> GPLGSMEQTEVLKPRTLADLIRILHQLFAGDEVNVEEVQAIMEAYESDPTEWAMYAKFDQYRYTRNLVDQGNGKFNLMILCWGEGHGSSIHDHTNSHCFLKMLQGNLKETLFAWPDKKSNEMVKKSERVLRENQCAYINDSIGLHRV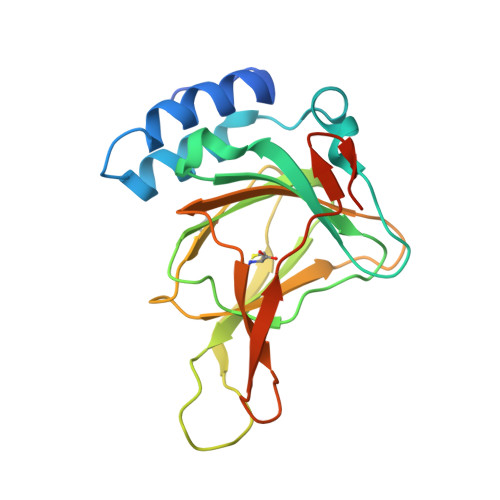ENISHTEPAVSLHLYSPPFDTCHAFDQRTGHKNKVTMTFHSKFGIRTPNATSGSLENN> MDQFECINVADAHQKLQEKEAVLVDIRDPQSFAMGHAVQAFHLTNDT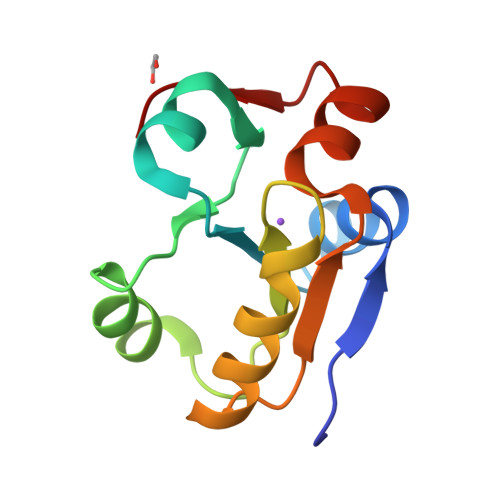LGAFMRDNDFDTPVMVMCYHGNSSKGAAQYLLQQGYDVVYSIDGGFEAWQRQFPAEVAYGA>[2x]NSFLQDVPYWMLQNRSEYITQGVDSSHIVDGKKTEEIEKIATKRATIRVAQNIVHKLKEAYLSKTNRIKQKITNEMFIQMTQPIYDSLMNVDRLGIYINPNNEEVFALVRARGFDKDALS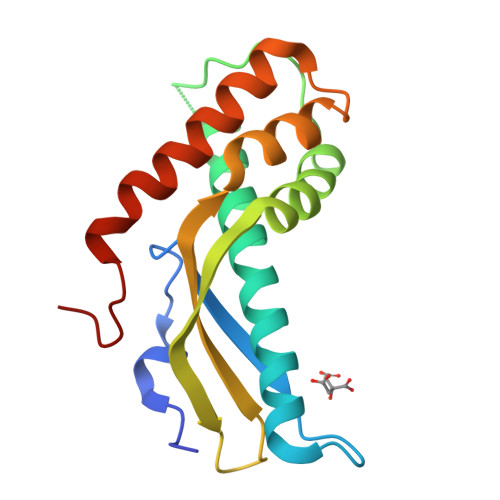EGLHKMSLDNQAVSILVAKVEEIFKDSVNYGDVKVPIAM>[2x]GAMDLLELSDVDSESSDISQPYVVCRQCPEYRRQAAQPPHCPAPEGEPGAPQALGDAPSTSVSLTTAVQDYVCPLQ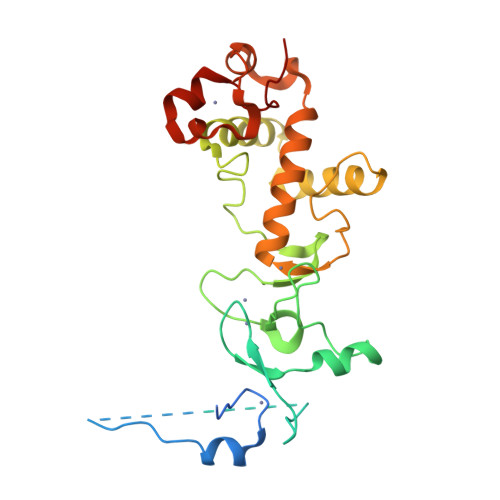GSHALCTCCFQPMPDRRVEREQDPRVAPQQCAVCLQPFCHLYWGCTRTGCYGCLAPFCELNLGDKCLDGVLNNNSYESDILKNYLATRGLTWKNMLTESLVALQRGVFLLSDYRVTGDTVLCYCCGLRSFRELTYQYRQNIPASELPVAVTSRPDCYWGRNCRTQVKAHHAMKFNHICEQTRFKN>[2x]MHHHHHHENLYFQGAASSHKLAEANTDFAFSLYRELAKSSPDKNIFFSPVSISSALAMLSLGAKGDTHTQILEGLGFNSEADIHQGFQHLLQTLNRPKGLQLKTANGLFVDKSLKLLDSFLEDSKKLYQAEAFSVDFDPEEAKKQINDWVEKQTNGKIKDLLKDLDSDTVLVLVNAIYFKGKWKKPFDPENTKEEDFHVDEKTTV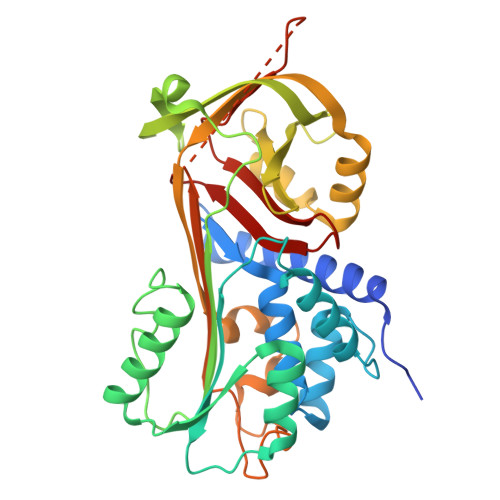KVPMMSQKGKFYYYHDDELSCKVLELPYKGNASMLIILPDEGGLQHLEQSLTPETLSKWLKSLTRRSVELYLPKFKIEGTYDLKEVLSNLGITDLFSPGADLSGITEEKLYVSKAVHKAVLEVNKEGTEAAAATGVEIVPRSPPEFKADRPFLFLIRENKTGSILFMGKVVNP>GSHEVKREYKEMEGSPEIKSKRRQFHQEL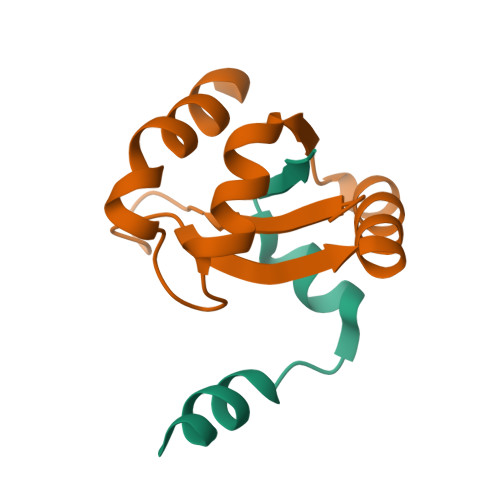QSSNLRADVRRSSVIVANPTHVAIGIRYRRGETPLPLVTLKHTDALALRVRRIAEEEGIPVLQRIPLARALLRDGNVDQYIPADLIQATAEVLRWLE[2x]>[4x]MSKINVNVENVSGVQGFLFHTDGK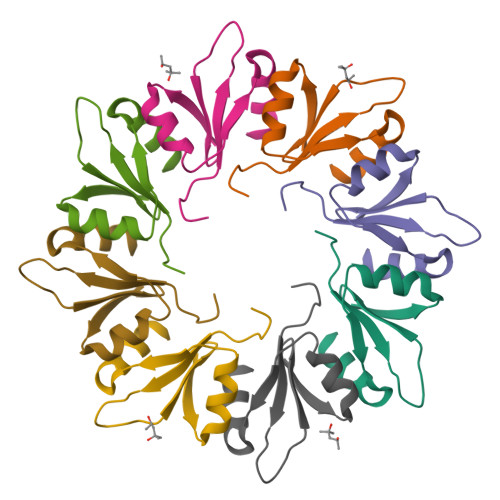ESYGYRAFINGVEIGIKDIETVQGFQQIIPSINISKSDVEAIRKAMKK> GPMDQYKEEDSTVSILPTSLPQIHRANMLAQGSPAASKISPLVTKKSKTRWHFGIRSRSYPLDVMGEIYIALKNLG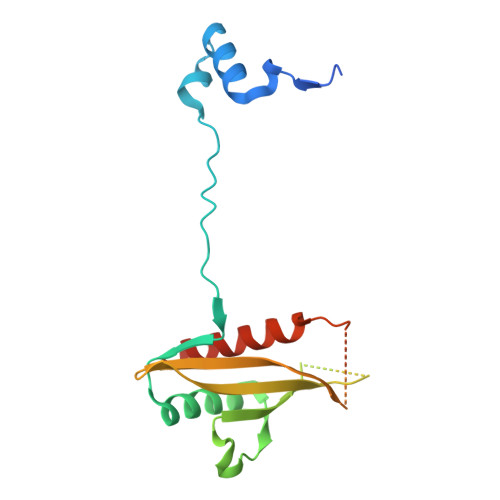AEWAKPSEEDLWTIKLRWKYDIGNKTNTNEKIPDLMKMVIQLFQIETNNYLVDFKFDGWESSYGDDTTVSNISEDEMSTFSAYPFLHLTTKLIMELAVNSQSN>MGVDP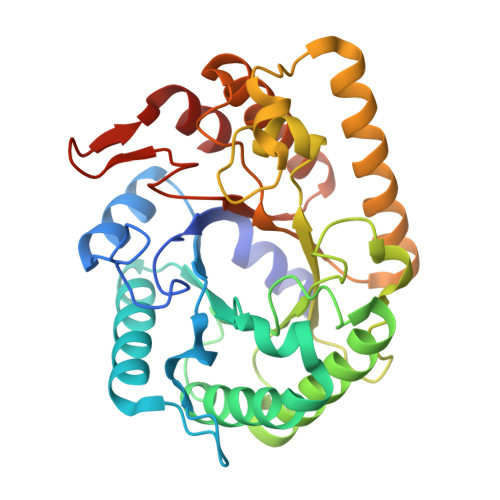FERNKILGRGINIGNALEAPNEGDWGVVIKDEFFDIIKEAGFSHVRIPIRWSTHAYAFPPYKIMDRFFKRVDEVINGALKRGLAVVINIHHYEELMNDPEEHKERFLALWKQIADRYKDYPETLFFEILNEPHGNLTPEKWNELLEEALKVIRSIDKKHTIIIGTAEWGGISALEKLSVPKWEKNSIVTIHYYNPFEFTHQGAEWVEGSEKWLGRKWGSPDDQKHLIEEFNFIEEWSKKNKRPIYIGEFGAYRKADLESRIKWTSFVVREMEKRRWSWAYWEFCSGFGVYDTLRKTWNKDLLEALIGGDSIE[2x]5,6,7,8-TETRAHYDRO[1]BENZOTHIENO[2,3-D]PYRIMIDIN-4(3H)-ONE 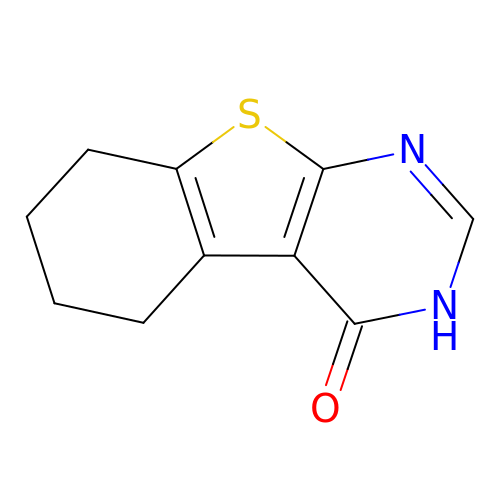| C10 H10 N2 O S | NMMOEJUJKIXUQZ-UHFFFAOYSA-N> XNWKLLAKGLLIRE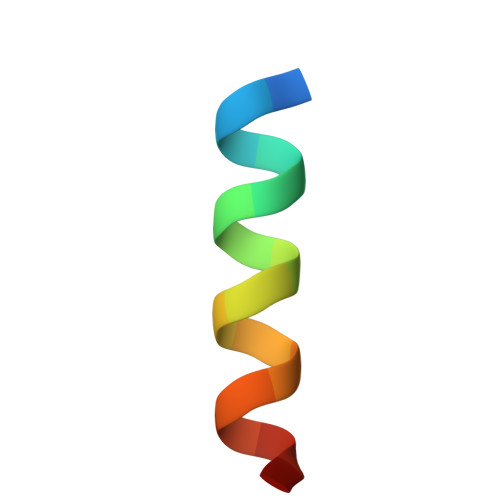RLKR> MDKDMHINEIVLRGCAPTPLAAYLKALGVLRLVCEQVDATAKGWWQDECFMLRTRLDDNDLRRFFIEDYRPTPMLSPWNGGSGFYRKGNETAWSTLEKIITTQAERWRPFRDTAEVMADALEHLKLTEKPAELDKRALLARLRATLDDEFLPWLDAAVLLTDDKPDYPPLLGTGGNDGRLDFTSNYMQRLLEMFDPVTGKAQGDVGNKLESALFARPVPGMTALAIGQFSPGAAGGPNSSTGFDSGAQVNIWDYVLMLEGALLFAATATRRLESADPSALSYPFTVRPSGGGSGAVALGDERPARAEIWMPLWERP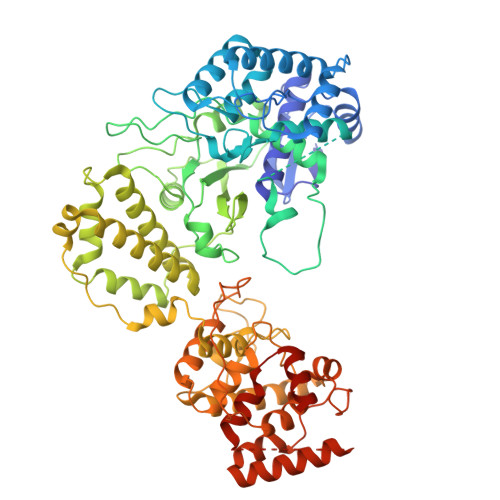ASLPELRVLLGEGRVTLNGRLPRDGLDFARAVAKLGTDRGVRAFQRYAFMMRSGKAYLATPLNRFHVHRNPKADLIDQLERGDWLRRFRRAARSTHAPARLQGLAHRLDDALFDLVRVADPRRVQEVLKVLGEVQFYLALSPSLREQVRPVPRLDAHWVEAARDDSHEFRVAAALAGLDDGLPMGVHLAPIDPVKRNVWAPESRLAVWGQGNLSDNLAQVLQRRLLTASRTDLNDKPLSGRCPADEGAVAAFLAGDADERRIAELMAGLACARLPARLPLRQRGASEASSLPMIYALLKPLFVPDAQLREAAVLTPDGCLPLPPALPRLLRAGPAGVGRAVDLARRRRRASGLADAGWRLTPPYPDGGRLLAALMIPVEIRVIKGFIKRLADHKSDEPATQDAS> MRMFKITACVPSQTR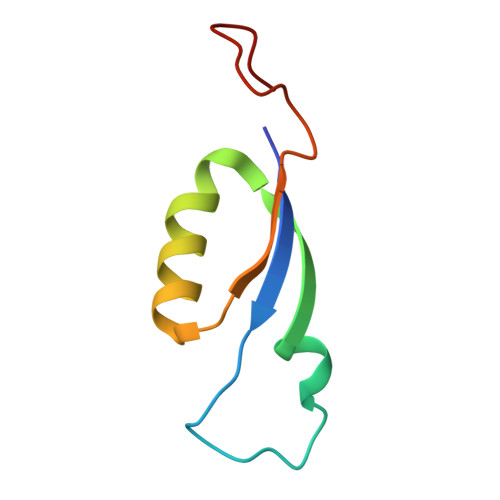IRTQRELQNTYFTKLVPYENWFREQQRIQKMGGKIVKVELFTGKPGVNTGLA>[60x]GPM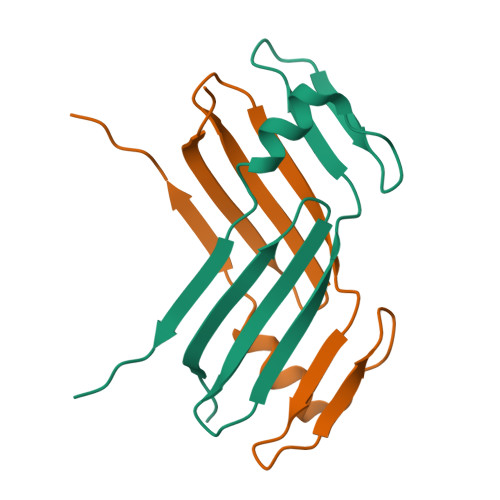GSAQLLKSVFVKNVGWATQLTSGAVWVQFNDGSQLVVQAGVSSISYTSPNGQTTRYGENEKLPDYIKQKLQCLSSILLMFSNPTPNFH The biocatalytic reduction of the oxime moiety to the corresponding amine group has only recently been found to be a promiscuous activity of ene-reductases transforming α-oximo β-keto esters. By studying the crystal structures of enzyme oxime complexes, analyzing molecular dynamics simulations, and investigating biocatalytic cascades and possible intermediates, we obtained evidence that the reaction proceeds via an imine intermediate and not via the hydroxylamine intermediate. To gain more insight into the reaction pathway, we determined the crystal structures of the two enzymes OPR3 and XenA in complex with the oxime substrates 1a–c, either by co-crystallization or by soaking. All the crystal structures obtained had a high resolution (1.9–1.35 Å) and showed clear electron density features for the oximes.

In general, XenA structures showed a better-defined electron density for the substrate when prepared by soaking, while for OPR3, clearer results were obtained by co-crystallization. The propanoyl moiety of oxime 1b points into this cavity and is likely stabilized by hydrophobic interactions. Substrates with an acetyl moiety (such as oximes 1a and 1c) give the non-productive binding mode described above. Comparable experimental pKa values are reported for chemically similar oximes and for the 8-hydroxycoumarin and para-hydroxybenzaldehyde. Substrates of ene-reductases usually bind with the hydride-receiving atom within van der Waals distance from the N5 of the flavin and with an enzyme-dependent angle between the flavin N10–N5 axis and the atom receiving the hydride. In the cases mentioned above, none of these criteria are satisfied, and the binding modes very likely correspond to catalytically non-active complexes. Thus, we will refer to it as the “non-productive binding mode”. Remarkably, a non-canonical tyrosine residue was found to contribute to the catalytic activity of the ene-reductase OPR3, protonating the hydroxyl group of the oxime in the first reduction step. Comparison with the other previously investigated enzymes revealed that this tyrosine is structurally conserved, though in class I/II OYEs, it is located close to the C-terminus of the enzyme (Y370 in OPR3). For OPR3, a non-canonical tyrosine residue was suggested as potentially catalytically relevant for the transformation of oxime substrates.

>HHHHHHMASSAQDGNNPLFSPYKMGKFNLSHRVVLAPMTRCRALNNIPQAALGEYYEQRATAGGFLITEGTMISPTSAGFPHVPGIFTKEQVREWKKIVDVVHAKGAVIFCQLWHVGRASHEVYQPAGAAPISSTEKPISNRWRILMPDGTHGIYPKPRAIGTYEISQVVEDYRRSALNAIEAGFDGIEIHGAHGYLIDQFLKDGINDRTDEYGGSLANRCKFITQVVQAVVSAIGADRVGVRVSPAIDHLDAMDSNPLSLGLAVVERLNKIQLHSGSKLAYLHVTQPRYVAYGQTEAGRLGSEEEEARLMRTLRNAYQGTFICSGGYTRELGIEAVAQGDADLVSYGRLFISNPDLVMRIKLNAPLNKYNRKTFYTQDPVVGYTDYPFLQGNGSNGPLSRL[2x]> IIGGSDADIKNFPWQVFFDNPWAGGALINEYWVLTAAHVVEGNREPTMYVGSTSVQTSRLAKSK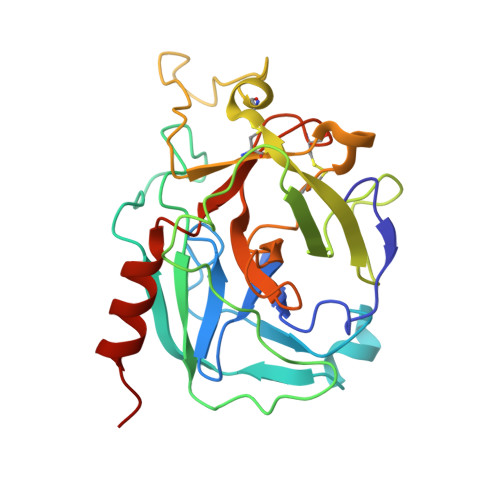MLTPEHVFIHPGWKLLEVPEGRTNFDNDIALVRLKDPVKMGPTVSPICLPGTSSDYNLMDGDLGLISGWGRTEKRDRAVRLKAARLPVAPLRKCKEVKVEKPTADAEAYVFTPNMICAGGEKGMDSCKGDAGGAFAVQDPNDKTKFYAAGLVSWGPQCGTYGLYTRVKNYVDWIMKTMQENSTPRED>[2x]GSP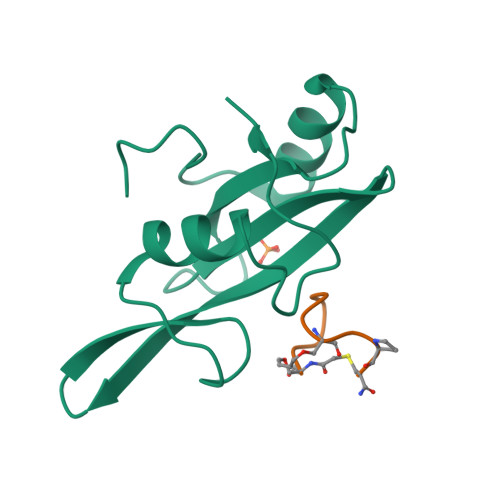ASGTSLSAAIHRTQLWFHGRISREESQRLIGQQGLVDGLFLVRESQRNPQGFVLSLCHLQKVKHYLILPSEEEGRLYFSMDDGQTRFTDLLQLVEFHQLNRGILPCLLRHCCTRVAL;>[2x]SFEGYDNXFPX>[6x]MKDFLRLELPVLPLRNTVVLPHTTTGVDVGRLKSKRAVEEALSADRLLFLVTQKDPEVDDPAPEDLYAVGTLAVVKQAMRLPDGTLQVMVEARSRARLLSYVAAPYLRAVGEAIPEPPLKD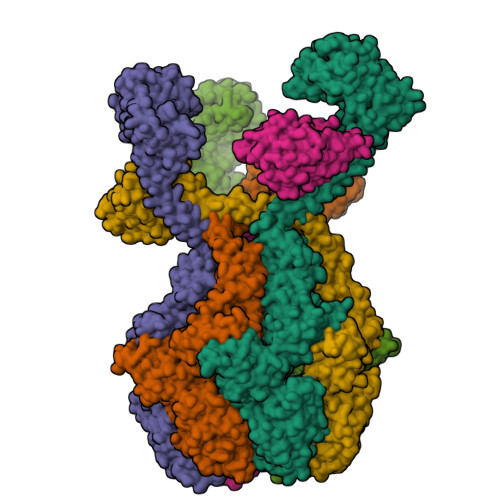PELARVLVNEVQEAFERYLQNHKTLRLDRYQQEAVKSTRDPAILADLVAHHATWTLEEKQTILETPEVEERLKRVLALLLRDLERFELDKKIAARVKEQMDQNQREYYLREQMKAIQKELGGGEDFLTEIEELRERIEKKGMPEPVKEKALKELKRLERMQPGSPEATVSRTYLDWLLEVPWTEADPEVLDISVTKRVLDEDHYGLKEVKERILEYLAVRQLTQGKEVKGHAPILCFVGPPGVGKTSLGKSIARSMNRRFHRISLGGVRDEAEIRGHRRTYIGALPGKIIQGMKQVGVVNPVFLLDEIDKLSSDWRGDPAAALLEVLDPEQNHTFTDHYLDVPYDLSKVFFITTANTLSTIPRPLLDRMEVIEIPGYTLHEKRAIARYFRWPFQVKEAGLEGRLEITDRAIERIVQEYTREAGVRNLDRELSKVARKAAKDYLEKPWEGVRVVDAEDLEAYLGVPKYRPDRAEKEPQVGAAQGLAWTPYGGTLLTIEAVAVPGTGKVNLTGNLGEVMKESAHAALTYLRAHREEWGLPEGFHKDYDLHIHVPEGATPKDGPSAGITIATALASALTGRPVRMDIAMTGEITLRGRVLPIGGVKEKLLAAHQAGIHRVILPKENAAELKEVPEEILKDLEIHFVEEVGEVLKLLLLPPPPPPAVQPDRPQPGVGA> TSRPYACELCAKQFQSPSTLKMHMRCHTGEKPYQCKTCGRCFSVQGNLQKHERIHLGLKEFVCQYCNKAFTLNETLKIHERIHTGEKRYHCQ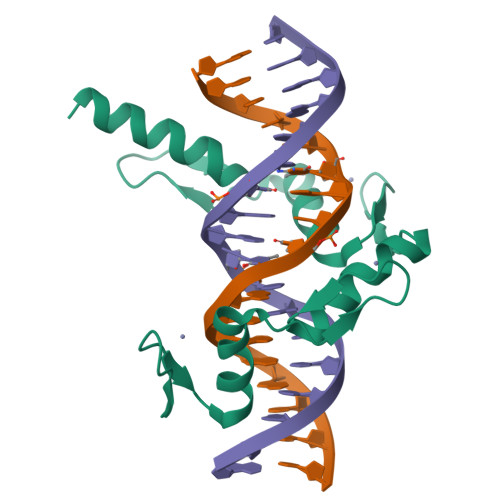FCFQRFLYLSTKRNHEQRHIREHNGKG>[2x]MREYKLVVLGSGGVGKSALTVQFVQGIFVEKYD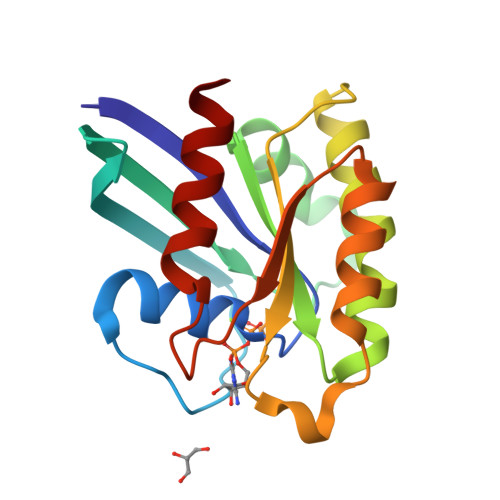PTIEDSYRKQVEVDAQQCMLEILDTAGTEQFAAMRDLYMKNGQGFALVYSITAQSTFNDLQDLREQILRVKDTDDVPMILVGNKCDLEDERVVGKEQGQNLARQWSNCAFLESSAKSKINVNEIFYDLVRQINR N-{(1S,2S)-1-[(2S)-4-benzyl-3-oxopiperazin-2-yl]-1-hydroxy-3-phenylpropan-2-yl}-7-ethyl-1,3,3-trimethyl-2,2-dioxo-1,2,3,4-tetrahydro-2lambda~6~-[1,2,5]thiadiazepino[3,4,5-hi]indole-9-carboxamide 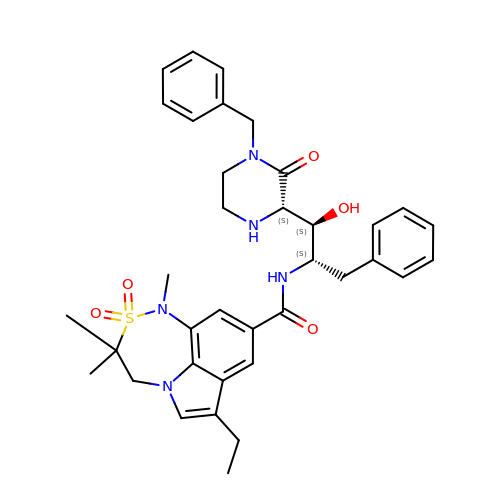| C36 H43 N5 O5 S | WBWSVNAKBNLSOJ-WXWREJFYSA-N>GAMGSEKSPSAQELKEQGNRLFVGRKYPEAAACYGRAITRNPLVAVYYTNRALCYLKMQQHEQALADCRRALELDGQSVKAHFFLGQCQLEMESYDEAIANLQRAYSLAKEQRLNFGDDIPSALRIAKKKRWNSIEERR[2x];>GIDPFTEFSLESYAFNMKATVEDEKLQGK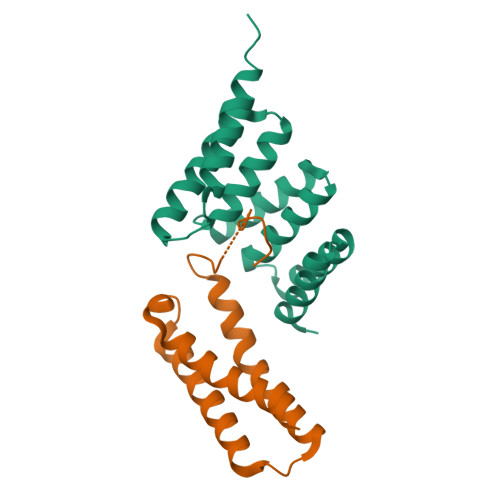INDEDKQKILDKCNEIINWLDKNQTAEKEEFEHQQKELEKVCNPIITKLYQSAGGMPGGMPGGFGPTIEEVD[2x]> MPKLVTWMNNQRVGELTKLANGAHTFKYAPEWLASRYARPLSLSLPLQRGNITSDAVFNFFDNLLPDSPIVRDRIVKRYHAKSRQPFDLLSEIGRDSVGAVTLIPEDETVTHPIMAWEKLTEARLEEVLTAYKADIPLGMIREENDFRISVAGAQEKTAL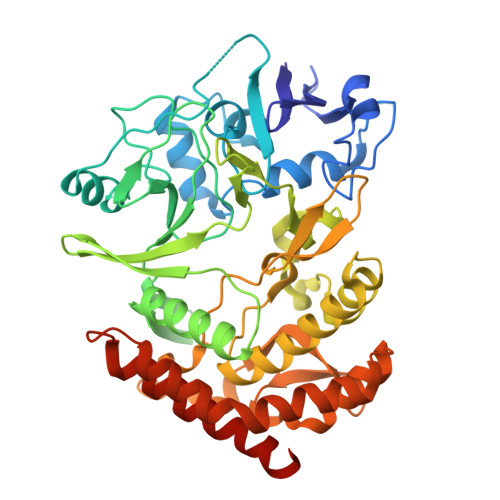LRIGNDWCIPKGITPTTHIIKLPIGEIRQPNATLDLSQSVDNEYYCLLLAKELGLNVPDAEIIKAGNVRALAVERFDRRWNAERTVLLRLPQEDMCQTFGLPSSVKYESDGGPGIARIMAFLMGSSEALKDRYDFMKFQVFQWLIGATDGHAKNFSVFIQAGGSYRLTPFYDIISAFPVLGGTGIHISDLKLAMGLNASKGKKTAIDKIYPRHFLATAKVLRFPEVQMHEILSDFARMIPAALDNVKTSLPTDFPENVVTAVESNVLRLHGRLSREYGSKHHHHHH> HEYAVGKIKIEHPWLRAPLEGETRAQLYMLVVNSADRPDRLIGVKSADFRSVQFHIAPHLVA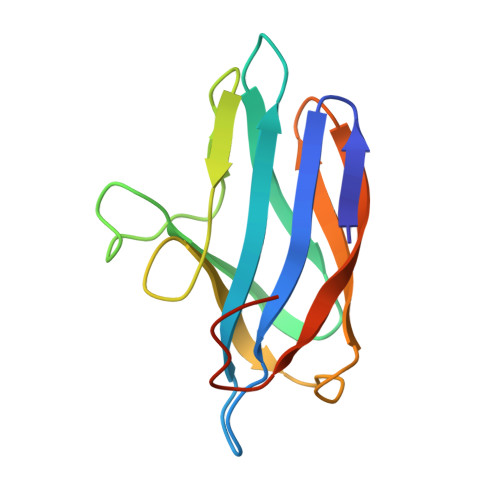REDAIYLPPLSRVTMAPGGSHVELVDISKMNPVGWAAEMTLVFEKAGEVTIDAAVEAPDAMHAHDAEAM Phosphopantetheinyl transferases (PPTases) are essential enzymes involved in primary and secondary metabolite biosynthetic pathways. They catalyze the transfer of the 4ʹ‐phosphopantetheinyl (Ppant) moiety of coenzyme A (CoA) to a strictly conserved serine residue of carrier protein (CP) domains present in fatty acid synthases (FASs), polyketide synthases (PKSs) and non-ribosomal peptide synthetases (NRPSs). The covalent attachment of the 20 Å-long Ppant arm to CP domains allows tethering substrates and chemical intermediates through a reactive thioester bond and transferring them to the different catalytic centers of the synthases where enzymatic modifications can proceed. Owing to their role in activating enzymes essential for bacterial viability and pathogenicity, phosphopantetheinyl transferases represent novel and attractive drug targets.

Despite the absence of inhibition on M. abscessus growth, and since 8918 was able to inhibit ACP conversion in our in vitro assay, we wanted to confirm binding to PptAb using X-ray crystallography. Crystals of PptAb prepared in the presence of CoA and Mn2+ were soaked in a 5 mM solution of 8918 and the structure of the complex was solved at 1.40 Å. Interestingly, binding of compound 8918 to PptAb displays the same pattern as that observed for PptT. Three hydrogen bonds involving the catalytic base Glu153, one hydrogen bond formed with the main chain oxygen atom of Leu167, and van der Waals contacts established with Lys152, Tyr156, Lys157, Trp166, Gly168, Phe169, and CoA are found. It is noteworthy that a second 8918 molecule was found at the surface of PptT11, which is not the case for PptAb. We found that 8918 inhibits ACP conversion by PptAb at nM concentrations and that total inhibition was achieved in the µM range. The fact that the Ppant of CoA is perfectly ordered in the structure of the complex with PcpS, which is not the case for PptAb-CoA-8918 ± ACP complexes is in accordance with the finding that 8918 inhibits its target by displacing the Ppant arm, which decreases but does not abolish catalytic activity in the case of PptT11. Indeed, unlike M. tuberculosis for which the MIC90 of compound 8918 varies from 0.56 to 3 μM on clinical isolates, it has no impact on the growth of M. abscessus in broth culture at concentrations up to 128.0 μM, probably as a result of its inability to penetrate the cell envelope.

> MPVTDQLIASVVPELLPSAELYEDPPGLEPLPEEEPLIAKSVAKRRNEFITVRYCARQALSVLGIPEVPILKGDKGQPLWPDGIVGSMTHTEGFRGAVVGRTGEVRSVGIDAEPHDVLPNGVLKSIALPVERDELDALPAGTHWDRLLFCAKETTYKAWFPLTARWLGFEDAHITIDPDGTFTSRILVDGRANDGTVLSAFDGRWIIDKGLILTAIVVPKLAAALEHHHHHH>MSTQKNARATAGEVEGSDALRMDADRAEQCVDALNADLANVYVLYHQLKKHHWNVEGAEFRDLHLFLGEAAETAEEVADELAERVQALGGVPHASPETLQAEASVDVEDEDVYDIRTSLANDMAIYGDIIEATREHTELAENLGDHATAHMLREGLIELEDDAHHIEHY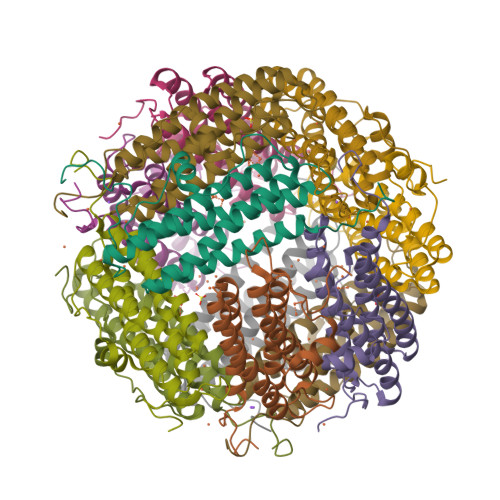LEDDTLVTQGALE[4x]> SYSS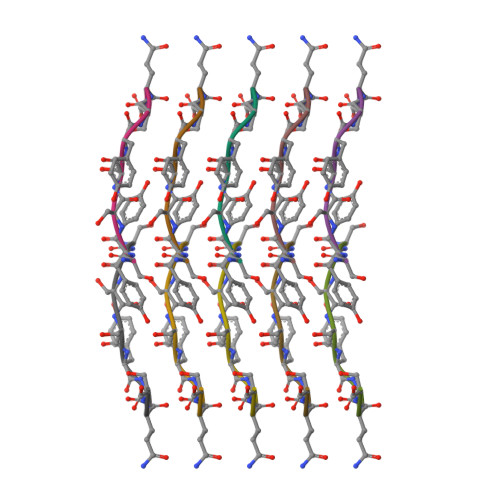YGQS>MVPISPIETVPVKLKPGMDGPKVKQWPLTEEKIKALVEICTEMEKEGKISKIGPENPYNTPVFACKKKDSTKWRKLVDFRELNKRTQDFWEVQLGIPHPAGLKKKKSVTVLDVGDAYFSVPLDEDFRKYTAFTIPSINNETPGIRYQYNVLPQGWKGSPAIFQSSMTKILEPFKKQNPDIVIYQYMDDLYVGSDLEIGQHRTKIEELRQHLLRWGLTTPDKKHQKEPPFLWMGYELHPDKWTVQPIVLPEKDSWTVNDIQKLVGKLNWASQIYPGIKVRQLSKLLRGTKALTEVIPLTEEAELELAENREILKEPVHGVYYDPSKDLIAEIQKQGQGQWTYQIYQEPFKNLKTGKYARMRGAHTNDVKQLTEAVQKITTESIVIWGKTPKFKLPIQKETWETWWTEYWQATWIPEWEFVNTPPLVKLWYQLEKEPIVGAETFYVDGAANRETKLGKAGYVTNKGRQKVVPLTNTTNQKTELQAIYLALQDSGLEVNIVTDSQYALGIIQAQPDKSESELVNQIIEQLIKKEKVYLAWVPAHKGIGGNEQVDKLVSA[2x];>MAHHHHHHALEVLFQGPISPIETVPVKLKPGMDGPKVKQWPLTEEKIKALVEICTEMEKEGK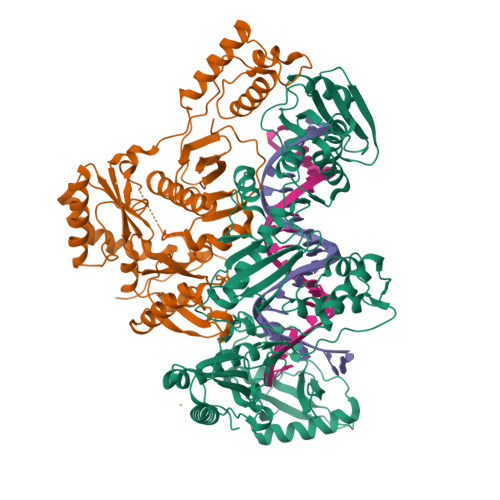ISKIGPENPYNTPVFAIKKKDSTKWRKLVDFRELNKRTQDFWEVQLGIPHPAGLKKKKSVTVLDVGDAYFSVPLDEDFRKYTAFTIPSINNETPGIRYQYNVLPQGWKGSPAIFQSSMTKILEPFKKQNPDIVIYQYMDDLYVGSDLEIGQHRTKIEELRQHLLRWGLTTPDKKHQKEPPFLWMGYELHPDKWTVQPIVLPEKDSWTVNDIQKLVGKLNWASQIYPGIKVRQLSKLLRGTKALTEVIPLTEEAELELAENREILKEPVHGVYYDPSKDLIAEIQKQGQGQWTYQIYQEPFKNLKTGKYARMRGAHTNDVKQLTEAVQKITTESIVIWGKTPKFKLPIQKETWETWWTEYWQATWIPEWEFVNTPPLVKLWYQ[2x]> GHMGAASASLAIGGVVIIGGGGHAKVVIESLRACGETVAAIVDADPTRRAVLGVPVVGDDLALPMLREQGLSRLFVAIGDNRLRQKLGRKARDHGFSLVNAIHPSAVVSPSVRLGEGVAVMAGVAINADSWIGDLAIINTGAVVDADCRLGAACHLGPASALAGGVSVGERAFLGVGAR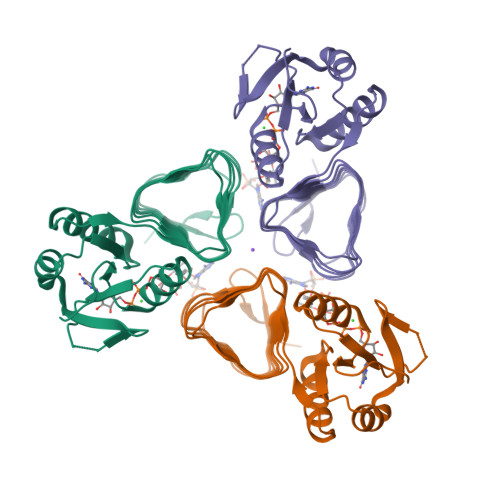VIPGVTIGADTIVGAGGVVVRDLPDSVLAIGVPAKIKGDRS>[3x]FSIAVTGATGQLGGLVIQHLMAAVPASQIIAIVRNVEKASTLADQGVEVRHGDYNQPESLQKAFAGVSKLLFISGPHYDNTLLIVQHANVVKAARDAGVKHIAYTGYAFAEESIIPLAHVHLATEYAIRTTNIPYTFLRNALYTDFFVNEGLRASTESGAIVTNAGSGIVNSVTRNELALAAATVLTEEGHENKTYNLVSNQPWTFDELAQILSEVSGKKVVHQPVSFEEEKNFMVNAGVPEPFAEITAAIYDAISKGEASKTSDDLQKLIGSLTPLKETVKQALKM;> FSIAVTGATGQLGGLVIQHLMAAVPASQIIAIVRNVEKASTLADQGVEVRHGDYNQPESLQKAFAGVSKLLFISGPHYDNTLLIVQHANVVKAARDAGVKHIAYTGYAFAEESIIPLAHVHLATEYATRTTNIPYTFLRNALYTDFFVNE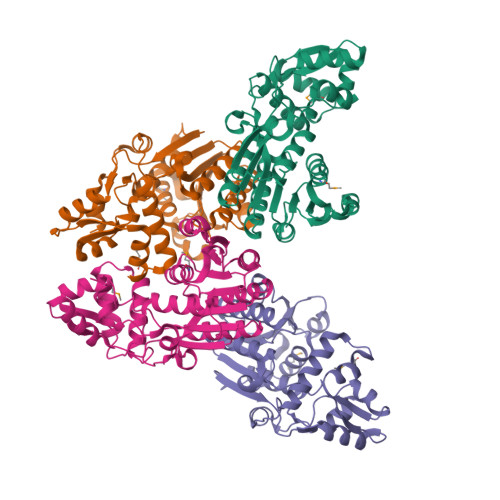GLRASTESGAIVTNAGSGIVNSVTRNELALAAATVLTEEGHENKTYNLVSNQPWTFDELAQILSEVSGKKVVHQPVSFEEEKNFMVNAGVPEPFAEITAAIYDAISKGEASKTSDDLQKLIGSLTPLKETVKQALKM thieno[3,2-b]thiophene-5-carboxylic 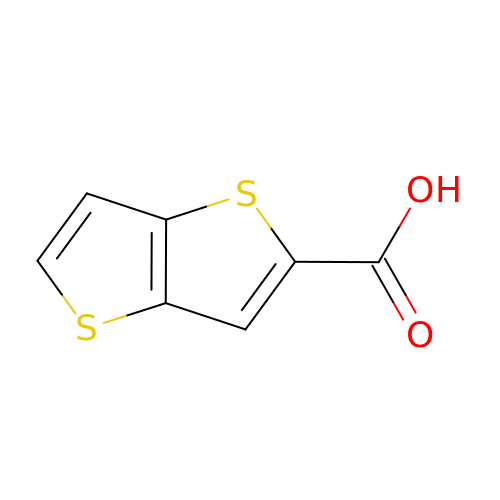acid | C7 H4 O2 S2 | GVZXSZWCZGKLRS-UHFFFAOYSA-N> MVPMDKTLKEFGADVQWDDYAQLFTLIKDGAYVKVKPGAQTAIVNGQPLALQVPVVMKDNKAWVSDTFINDVFQSGLDQTFQVEKRPHPLNALTADEIKQAVEIVKASADFKPNTRFTEISLLPPDKEAVWAFALENKPVDQPRKADVIMLDGKHIIEAVVDLQNNKLLSWQPIKDAHGMVLLDDFASVQNIINNSEEFAAAVKKRGITDAKK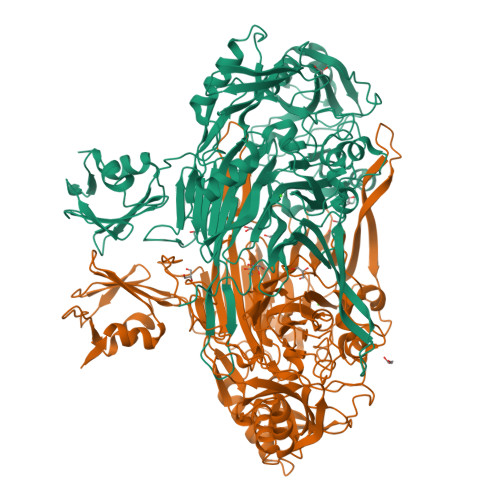VITTPLTVGYFDGKDGLKQDARLLKVISYLDVGDGNYWAHPIENLVAVVDLEQKKIVKIEEGPVVPVPMTARPFDGRDRVAPAVKPMQIIEPEGKNYTITGDMIHWRNWDFHLSMNSRVGPMFSTVTYNDNGTKRKVMYEGSLGGMIVPYGDPDIGWYFKAYLDSGDYGMGTLTSPIARGKDAPSNAVLLNETIADYTGVPMEIPRAIAVFERYAGPEYKHQEMGQPNVSTERRELVVRWISTVGNYDYIFDWIFHENGTIGIDAGATGIEAVKGVKAKTMHDETAKDDTRYGTLIDHNIVGTTHQHIYNFRLDLDVDGENNSLVAMDPVVKPNTAGGPRTSTMQVNQYNIGNQQDAAQKFDPGTIRLLSNPNKENRMGNPVSYQIIPYAGGTHPVAKGAQFAPDEWIYHRLSFMDKQLWVTRYHPGERFPEGKYPNRSTHDTGLGQYSKDNESLDNTDAVVWMTTGTTHVARAEEWPIMPTEWVHTLLKPWNFFDETPTLGALK;> HMVPMDKTLKEFGADVQWDDYAQLFTLIKDGAYVKVKPGAQTAIVNGQPLALQVPVVMKDNKAWVSDTFINDVFQSGLDQTFQVEKRPHPLNALTADEIKQAVEIVKASADFKPNTRFTEISLLPPDKEAVWAFALENKPVDQPRKADVIMLDGKHIIEAVVDLQNNKLLSWQPIKDAHGMVLLDDFASVQNIINNSEEFAAAVKKRGITDAKKVITTPLTVGYFDGKDGLKQDARLLKVISYLDVGDGNYWAHPIENLVAVVDLEQKKIVKIEEGPVVPVPMTARPFDGRDRVAPAVKPMQIIEPEGKNYTITGDMIHWRNWDFHLSMNSRVGPMFSTVTYNDNGTKRKVMYEGSLGGMIVPYGDPDIGWYFKAYLDSGDYGMGTLTSPIARGKDAPSNAVLLNETIADYTGVPMEIPRAIAVFERYAGPEYKHQEMGQPNVSTERRELVVRWISTVGNYDYIFDWIFHENGTIGIDAGATGIEAVKGVKAKTMHDETAKDDTRYGTLIDHNIVGTTHQHIYNFRLDLDVDGENNSLVAMDPVVKPNTAGGPRTSTMQVNQYNIGNQQDAAQKFDPGTIRLLSNPNKENRMGNPVSYQIIPYAGGTHPVAKGAQFAPDEWIYHRLSFMDKQLWVTRYHPGERFPEGKYPNRSTHDTGLGQYSKDNESLDNTDAVVWMTTGTTHVARAEEWPIMPTEWVHTLLKPWNFFDETPTLGALKK> MSAIPITPTKRIRRNLFDDAPATPPRPLKRKKLQFTDVTPESSPEKLQFGSQSIFLRTKALLQKSSELVNLNSSDGALPARTAEYEQVMNFLAKAISEHRSDSLYITGPPGTGKTAQLDMIIRQKFQSLPLSLSTPRSKDVLRHTNPNLQNLSWFELPDGRLES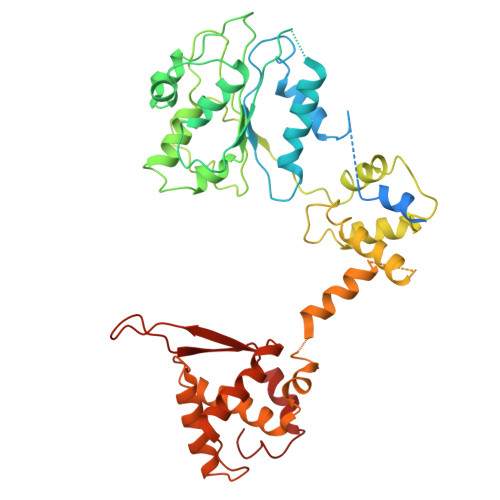VAVTSINCISLGEPSSIFQKIFDSFQDLNGPTLQIKNMQHLQKFLEPYHKKTTFVVVLDEMDRLLHANTSETQSVRTILELFLLAKLPTVSFVLIGMANSLDMKDRFLSRLNLDRGLLPQTIVFQPYTAEQMYEIVIQKMSSLPTIIFQPMAIKFAAKKCAGNTGDLRKLFDVLRGSIEIYELEKRFLLSPTRGSLNSAQVPLTPTTSPVKKSYPEPQGKIGLNYIAKVFSKFVNNNSTRTRIAKLNIQQKLILCTIIQSLKLNSDATIDESFDHYIKAITKTDTLAPLQRNEFLEICTILETCGLVSIKKTKCKGKTKRFVDKIDVDLDMREFYDEMTKISILKPFLH>[2x]RGSMSHYKSNVRDQVFNLFEVFGVDKVLGADKFSDLDADTAREMLTEIARLAEGPIAESF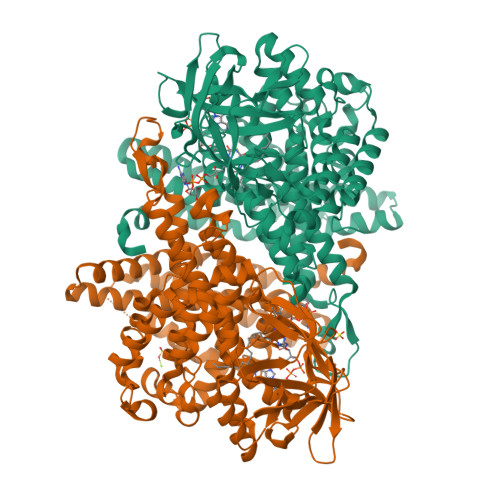VEGDRNPPVFDPETHTVTLPEGFKKSMRALFDGGWDKVGLAEHLGGIPMPRALQWALIEHILGANPAAYMYAMGPGMSEIFYNNGTDEQKKWATIAAERGWGATMVLTEPDAGSDVGAGRTKAVQQPDGTWHIEGVKRFITSADSDDLFENIMHLVLARPEGAGPGTKGLSLFFVPKFHFDHETGEIGERNGVFVTNVEHKMGLKVSATCELSLGQHGIPAVGWLVGEVHNGIAQMFDVIEQARMMVGTKAIATLSTGYLNALEYAKERVQGADMTQMTDKTAPRVTITHHPDVRRSLMTQKAYAEGLRAIYLYTATFQDAEVAQAVHGVDGDLAARVNDLLLPIVKGFGSETAYAKLTESLQTLGGSGFLQDYPIEQYIRDSKIDSLYAGTTAIQAQDFFFRKIIRDKGQALAYVAGEIEQFIKNENGNGRLKTERELLATALADVQGMAASLTGYLMAAQEDAASIYKVGLGSVRFLMAVGDLLSGWLLARQAAVAIEKLDAGATGADKSFYEGKIAAASFFAKNMLPLLTSTRQIIENLDNDVMELDEAAF>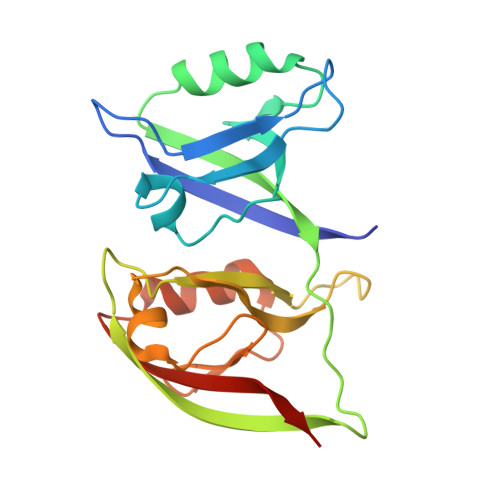 GPGSFKGSTVVELMKKEGTTLGLTVSGGIDKDGKPRVSNLRQGGIAARSDQLDVGDYIKAVNGINLAKFRHDEIISLLKNVGERVVLEVEYELPPVSIQGSSVMFRTVEVTLHKEGNTFGFVIRGGAHDDRNKSRPVVITCVRPGGPADREGTIKPGDRLLSVDGIRLLGTTHAEAMSILKQCGQEATLLIEYDVSVMDS> MGHSKQIRILLLNEMEKLEKTLFRLEQGYELQFRLGPTLQGKAVTVYTNYPFPGETFNREKFRSLDWENPTEREDDSDKYCKLNLQQSGSFQYYFLQGNEKSGGGYIVVDPILRVGADNHVLPLDCVTLQTFLAKCLGPFDEWESRLRVAKESGYNMIHFTPLQTLGLSRSCYSLANQLELNPDFSRPNRKYTWNDVGQLVEKLKKEWNVICITDVVYNHTAANSKWIQEHPECAYNLVNSPHLKPAWVLDRALWRFSCDVAEGKYKEKGIPALIENDHHMNSIRKIIWEDIFPKLKLWEFFQVDVNKAVEQFRRLLTQENRRVTKSDPNQHLTIIQDPEYRRFGCTVDMNIALTTFIPHDKGPAAIEECCNWFHKRMEELNSEKHRLINYHQEQAVNCLLGNVFYERLAGHGPKLGPVTRKHPLVTRYFTFPFEEIDFSMEESMIHLPNKACFLMAHNGWVMGDDPLRNFAEPGSEVYLRRELICWGDSVKLRYGNKPEDCPYLWAHMKKYTEITATYFQGVRLDNCHSTPLHVAEYMLDAARNLQPNLYVVAELFTGSEDLDNVFVTRLGISSLIREAMSAYNSHEEGRLVYRYGGEPVGSFVQPCLRPLMPAIAHALFMDITHDNECPIVHRSAYDALPSTTIVSMACCASGSTRGYDELVPHQISVVSEERFYTKWNPEALPSNTGEVNFQSGIIAARCAISKLHQELGAKGFIQVYVDQVDEDIVAVTRHSPSIHQSVVAVSRTAFRNPKTSFYSKEVPQMCIPGKIEEVVLEARTIERNTKPYRKDENSINGTPDITVEIREHIQLNESKIVKQAGVATKGPNEYIQEIEFENLSPGSVIIFRVSLDPHAQVAVGILRNHLTQFSPHFKSGSLAVDNADPILKIPFASLASRLTLAELNQILYRCESEEKEDGGGCYDIPNWSALKYAGLQGLMSVLAEIRPKNDLGHPFCNNLRSGDWMIDYVSNRLISRSGTIAEVGKWLQAMFFYLKQIPRYLIPCYFDAILIGAYTTLLDTAWKQMSSFVQNGSTFVKHLSLGSVQLCGVGKFPSLPILSPALMDVPYRLNEITKEKEQCCVSLAAGLPHFSSGIFRCWGRDTFIALRGILLITGRYVEARNIILAFAGTLRHGLIPNLLGEGIYARYNCRDAVWWWLQCIQ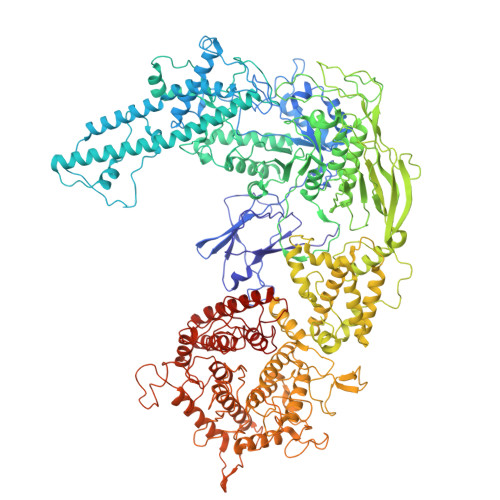DYCKMVPNGLDILKCPVSRMYPTDDSAPLPAGTLDQPLFEVIQEAMQKHMQGIQFRERNAGPQIDRNMKDEGFNITAGVDEETGFVYGGNRFNCGTWMDKMGESDRARNRGIPATPRDGSAVEIVGLSKSAVRWLLELSKKNIFPYHEVTVKRHGKAIKVSYDEWNRKIQDNFEKLFHVSEDPSDLNEKHPNLVHKRGIYKDSYGASSPWCDYQLRPNFTIAMVVAPELFTTEKAWKALEIAEKKLLGPLGMKTLDPDDMVYCGIYDNALDNDNYNLAKGFNYHQGPEWLWPIGYFLRAKLYFSRLMGPETTAKTIVLVKNVLSRHYVHLERSPWKGLPELTNENAQYCPFSCETQAWSIATILETLYDL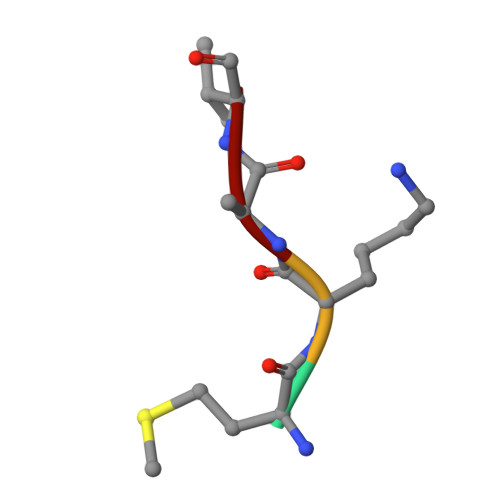> MKAV>GGDNVPYVTPLVRKLAEKHGVDLNTVTGTGIGGRIRKQDVLAAANGEAAPAEAAAPVSAWSTKSVDPEKAKLRGTTQKVNRIREITAMKTVEALQISAQLTQLHEVDMTRVAEL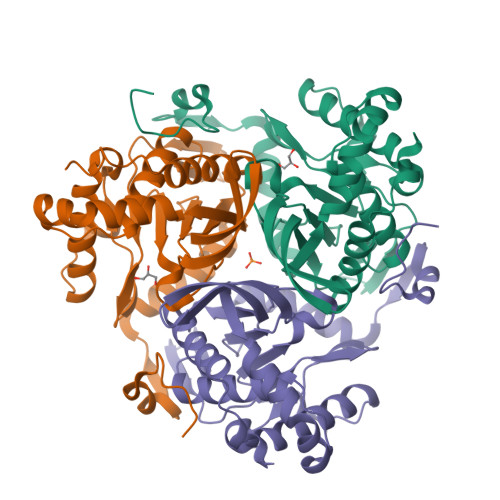RKKNKPAFIEKHGVNLTYLPFFVKAVVEALVSHPNVNASFNAKTKEMTYHSSVNLSIAVDTPAGLLTPVIHDAQDLSIPEIAKAIVDLADRSRNNKLKPNDLSGGTFTITNIGSEGALSDTPILVPPQAGILGTGAIVKRPVVITEDGIDSIAIRQMVFLPLTYDHQVVDGADAGRFLTTIKDRLETANFEGDLQL[3x]>MSEGEGQAKNRLFLGVDLGTSHTAVMSSRGKKFLLKSVVGYPKDVIGLKLLGRPYVVGDEAFEMRSYLDIRYPLQDGVLSEISDRDIEVARHLLTHVVKSAEPGPNDEICAVIGVPARASAANKALLLKMAQEVVHTALVVSEPFMVGYGLDKLINT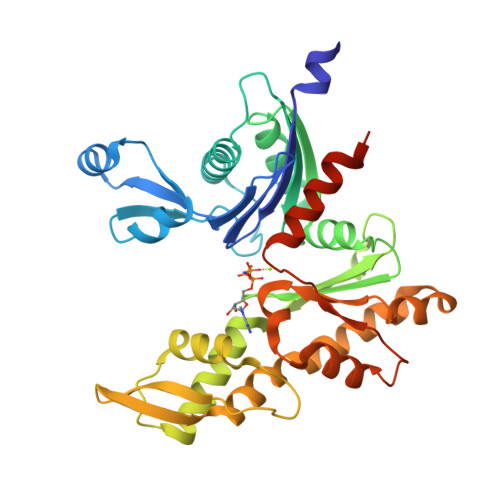IIVDIGAGTTDICALKGTVPGPEDQVTLTKAGNYVDERLQNAILERHPELQMNVNVACAVKEQFSFVGTPTEVASFEFRAAGKPVRADVTEPVKIACEALMPDIIESIETLLRSFQPEYQDTVLQNIVFAGGGSRIRGLAAYVKEKLRPFGDANVTCVKDPTFDGCRGALRLAEELPPQYWRQLGDVSGS[2x]>[4x]MVSKGEEDNMASLPATHELHIFGSINGVDFDMVGQGTGNPNEGYEELNLKSTKGDLQFSPWILVPHMGWGFHQYLPYPDGMSPFQAAMVDGS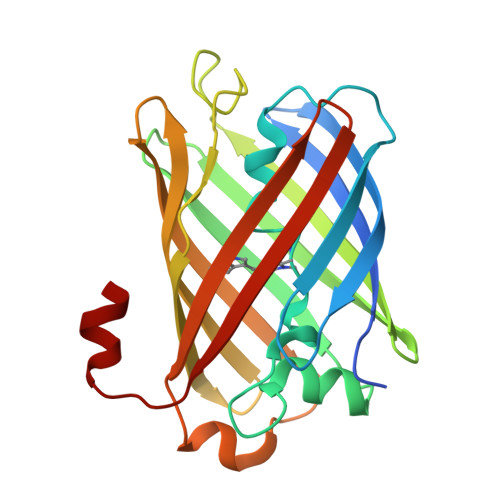GYQVHRTMQFEDGASLTVNYRYTYEGSHIKGEAQVKGTGFPADGPVMTNSLTAVDSCWSKKTYPNDKTIISTFKWSYTTGNGERYRSTARTTYTFAKPMAANYLKNQPVYVFRKDELKHSETELNFKEWQKAFTDVMGMDELYK>[2x]MHHHHHHAAGIPMNNPAIKRIGNHITKSPEDKREYRGLELANGIKVLLISDPTTDKSSAALDVHIGSLSDPPNIAGLSHFLQHMLFLGTKKYPKENEYSQFLSEHAGSSNAFTSGEHTNYYFDVSHEHLEGALDRFAQFFLSPLFDESAKDREVNAVDSEHEKNVMNDAWRLFQLEKATGNPKHPFSKFGTGNKYTLETRPNQEGIDVRQELLKFHSAYYSSNLMAVVVLGRESLDDLTNLVVKLFSEVENKNVPLPEFPEHPFQEEHLKQLYKIVPIKDIRNLYVTFPIPDLQKYYKSNPGHYLGHLIGHEGPGSLLSELKSKGWVNTLVGGQKAGARGFMFFIINVDLTEEGLLHVEDIILHMFQYIQKLRAEGPQEWVFQELKDLNAVAFRFKDKERPRGYTSKIAGILHYYPLEEVLTAEYLLEEFRPDLIEMVLDKLRPENVRVAIVSKSFEGKTDRTE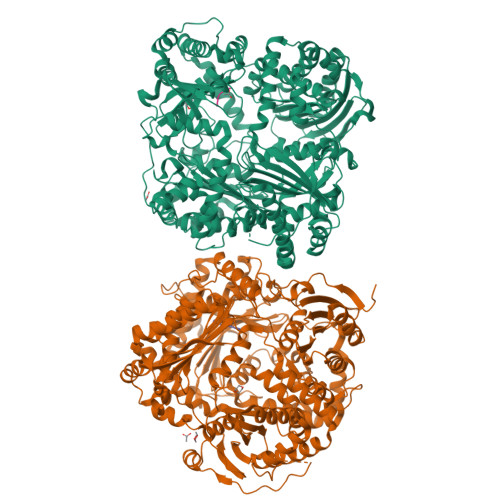EWYGTQYKQEAIPDAVIAKWQNAALNGKFKLPTKNEFIPTNFEILPLEAAATPYPALIKDTAMSKLWFKQDDKFFLPKANLNFEFFSPFAYVDPLHSNMAYLYLELLKDSLNEYAYAAELAGLSYDLQNTIYGMYLSVKGYNDKQPILLKKIIEKMATFEIDEARFEIIKEAYMRSLNNFRAEQPHQHAMYYLRLLMTEVAWTKDELKEALADVTLPRLKAFIPQLLSRLHIEALLHGNITKQAALGIMQMVEDTLIEHAHTKPLLPSQLAAYREVQLPDRGWFVYQQRNEVHNNSGIEIYYQTDMQSTSENMFLELFAQIISEPAFNTLRTKEQLGYIVFSGPRRANGIQGLRFIIQSEKPPHYLESRVEAFLITMEKSIEDMTEEAFQKHIQALAIRRLDKPKKLSAESAKYWGEIISQQYNFDRDNTEVAYLKTLTKADIIKFYKEMLAVDAPRRHKVSVHVLAREMDSNPVVGEFPAQNDINLSQAPALPQPEVIQNMTAFKRGLPLFPLVKPHINFMAAKL;>[2x]APPA>GAMPHDPSFTPTQLAARAAYLLRGNDLGTMTTAAPLLYPHMWSWDAAFVAIGLAPLSVERAVVELDTLLSAQWRNGMIPHIVFANGVDGYFPGPARWATATLADNAPRNRLTSGITQPPVHAIAVQRILEHARTRGRSTRAVAEAFLDRRWGDLMRWHRWLAECRDRNERGRITLYHGWESGMDNSPRWDSAYANVVPGKLPEYQRADNVIITDPSQRPSDGEYDRYLWLLEE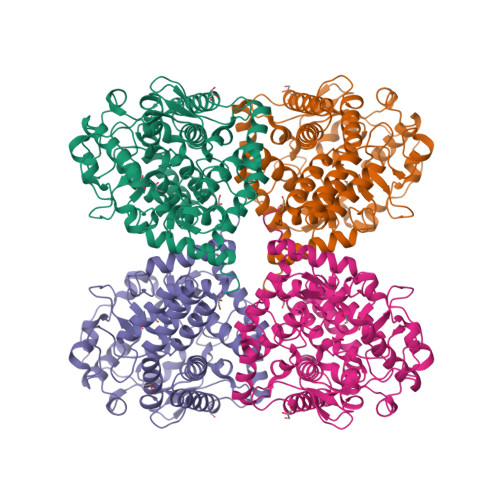MKAVRYDDERLPSVMSFQVEDVFFSAIFSVACQVLAEIGEDYKRPHADVKDLYLWAERFRAGVVETTDQRTGAARDFDVLAEKWLVTETAAQFAPLLCGGLPHDRERALLKLLEGPRFCGHPDLKYGLIPSTSPVSRDFRPREYWRGPVWPVLTWLFSWCFARRGWAERARLLRQEGLRQASDGSFAEYYEPFTGEPLGSMQFSWTAAAVLDWLG[2x]>[3x]MAEQLVEAPAYARTLDRAVEYLLSCQKDEGYWWGPLLSNVTMEAEYVLLCHILDRVDRDRMEKIRRYLLHEQREDGTWALYPGGPPDLDTTIEAYVALKYIGMSRDEEPMQKALRFIQSQGGIESSRVFTRMWLALVGEYPWEKVPMVPPEIMFLGKRMPLNIYEFGSWARATVVALSIVMSRQPVFPLPERARVPELYETDVPPRRRGAKGGGGWIFDALDRALHGYQKLSVHPFRRAAEIRALDWLLERQAGDGSWGGIQPPWFYALIALKILDMTQHPAFIKGWEGLELYGVELDYGGWMFQASISPVWDTGLAVLALRAAGLPADHDRLVKAGEWLLDRQITVPGDWAVKRPNLKPGGFAFQFDNVYYPDVCDTAVVVWALNTLRLPDE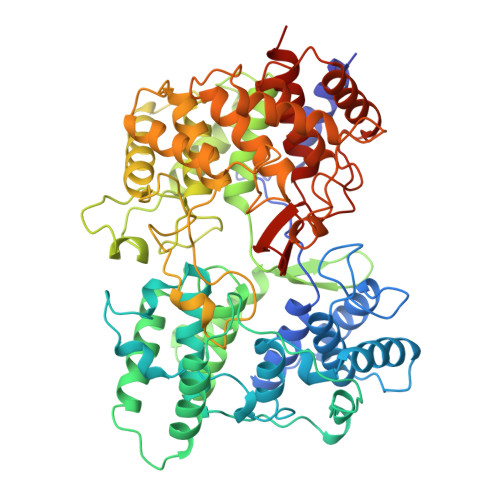RRRRDAMTKGFRWIVGMQSSNGGWGAYDVDNTSDLPNHIPFCDFGEVTDPPSEDVTAHVLECFGSFGYDDAWKVIRRAVEYLKREQKPDGSWFGRWGVNYLYGTGAVVSALKAVGIDTREPYIQKALDWVEQHQNPDGGWGEDCRSYEDPAYAGKGASTPSQTAWALMALIAGGRAESEAARRGVQYLVETQRPDGGWDEPYYTGTGFPGDFYLGYTMYRHVFPTLALGRYKQAIERR> UGCUCCUAGUACG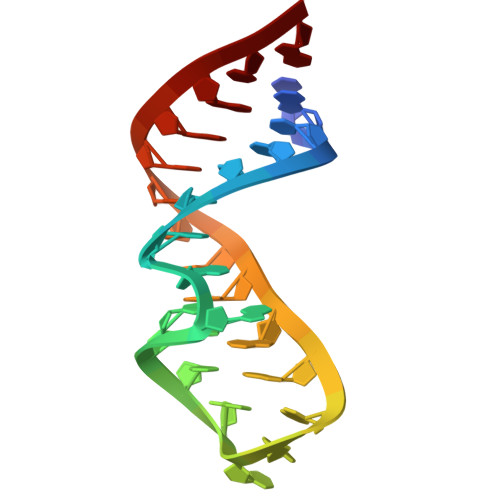UAAGGACCGGAGUG>MRGKIYDRNGKVLAEDVERYKLVAVIDKKASANSKKPRHVVDKKETAKKLSTVINMKPEEIEKRLSQKKAFQIEFGRKGTNLTYQDKLKIEKMNLPGISLLPETERFYPNGNFASHLIGRAQKNPDTGELKGALGVEKIFDSYLSGSKGSLRYIHDIWGYIAPNTKKEKQPKRGDDVHLTIDSNIQVFVEEALDGMVERYQPKDLFAVVMDAKTGEILAYSQRPTFNPETGKDFGKKWANDLYQNTYEPGSTFKSYGLAAAIQEGAFDPDKKYKSGHRDIMGSRISDWNRVGWGEIPMSLGFTYSSNTLMMHLQDLVGADKMK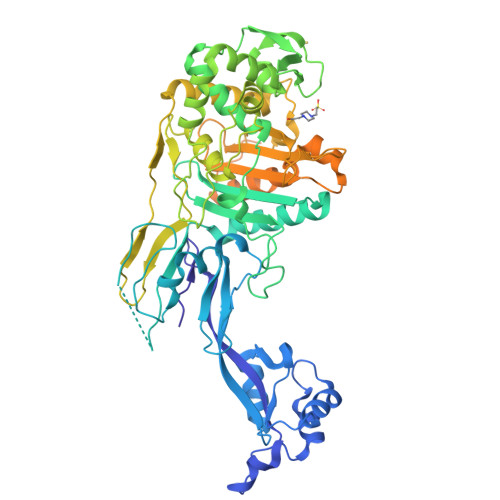SWYERFGFGKSTKGMFDGEAPGQIGWSNELQQKTSSFGQSTTVTPVQMLQAQSAFFNDGNMLKPWFVNSVENPVSKRQFYKGQKQIAGKPITKDTAEKVEKQLDLVVNSKKSHAANYRIDGYEVEGKTGTAQVAAPNGGGYVKGPNPYFVSFMGDAPKKNPKVIVYAGMSLAQKNDQEAYELGVSKAFKPIMENTLKYLNVGKSKDDTSNAEYSKVPDVEGQDKQKAIDNVSAKSLEPVTIGSGTQIKAQSIKAGNKVLPHSKVLLLTDGDLTMPDMSGWTKEDVIAFENLTNIKVNLKGSGFVSHQSISKGQKLTEKDKIDVEFSS[12x]> MSFLTSLTVAGKDYKVLNVSYDLAQETDASGRPSTVTRGGRIMIEVESTGST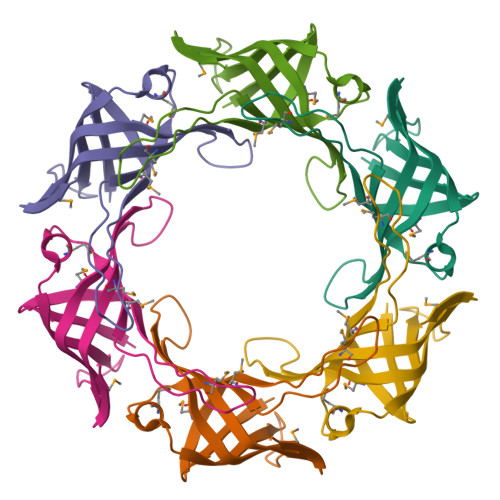ELFEWMTNNFERKDGSVKFIKRDSNATLKELKFTEAYMVKYKENFDHNSENPLTETFMISARKISMGGGEFDNAWVLEHHHHHH> MQNLEAQVTGSLVAFPDVTQKALKEDEINLDSVLRGKFSTGRTSLAWLACGPQLEITNSVTGERISAYHFSGLTERPPVVVAVKEFTWQKKTGLLVGLVEAEGSVLCLYDIGISKVVKAVVLPGSVTAVEPIINHGGASASTQHLHQSLRWFFGVTAVVTDVGHVLLIDLCLDEVSSNQDELDASDLEVMSVIPTKIPKLREAATRERRHLCLQLAAPTGTTVSCLSYISRTNQLAVGYSDGYFSLWNMKTLRRDYHVQIEGGRVPVCAVAFQEPENDPRNCCYLWAVQSSESGGDVSLHLLQLAFSDRKCLASGQIMYELLEYCEERYSLDLSGSTLSLRGQSNNTKLLGCQTIEKFRVHGEREDGVHEVTSPDTSVSVFSWQVNTYGQGKPSVYLGVFDINRWYQAQMPDSLRSGQFLRNCSYFAFWSLEAVVNITTQDIIFDILVHERSLSRGIPPSYPPPEQFYYPSTYNFDATCLLNSGLIHFACTGFQKETLHFLKKSGSSLNEAIPDGYNRCLAAGLLAPKFTDVQASSLSQEEQLQAILAAAVETSSLGLLTSCIKRWTAEEQPRSAANLRFVLEWTWKKVTLTKQEFDRLCFRLFDGSCNFIDPHTLQSLQQCHLYFSNLTAVLNCFIAQAKEVTQQGAVDLTNKQSVTRLLTLYASVVLWFCRSGMLPDSSDETVQLTRPFYNYQVIQQYYSDQRKKLERLARGKWDTSSLMIDGLINQFGDRIQQLWSRDDNGTGKYPPANLHALLDVYLLENADEMSKHAITIYFLLDIMYSFPDKPDSSIESFPTAFFVPGSLIKLIQGFWLLDHNDYQNSVDCILNPASSRVMSWQHSQIIENLLCHGDSRQALRYLQVMKPVATTSKEVKLHMTVLLANRSILEAWNLQRLHSSRLNVEELLKHMYEMCQEMGLIEELLKLTFTDFEQGYLHKFLQTTGVQNQELLLVHHLQRANYISALQLNQSLKTNHLNDCDRRLRERSGARNAILDQYGKILPRVQRTLASERAKPYSLPSLVWREVARPKPLSTTAKQAAPGSIITKANFICNVLSKIKEVSTANEKREEYSPYQSMVSEEPTAPPLQDIDVPDAFFGTPINKSRRVSRLLDSVVHPVLMEPTPLTSSDTDNNQTPHKSPLLKTSSPLHSSLRRIAHMRSFAKASEFSLLETPLVVRKAKALAANTASSGYTSITPQSILRSSVRTTPLVSPSVSPGRSLTPPLRPKETKISFMELSFTRHAKAAHSSEGNLLAISPVLRSSPDAVWSVKGKVASFTQNTPVKKLDEIDASSSGIQEESQDEMEVSKEISNISVRSEQASLEYHDAPTPEDLENDEISGTTNSQPQVNEVHHQMEDGQLTEKPAELALTEMQEEFIDSEEREIEYISAPLNGPNALECMTAVPDIYLEDASQCILETPEGSSVSVTGEQECVSSAKDSESVISIHDSDDAHSNLSENDQDSEEIEENNLRVPTTVTRCEEFDLIETKDLEVELEEADSEKTNYKDIYPDATVQLGFTVESIEQRYTCELADRRETPSETDEIEGEHFETENNFSLVLEGDVTEEEILEPSSSKTDLELTRPPIAHQKLISENRENIENCETTEKIPANMSPLVDSDHESKTLETLPSEADLSVAEKVLKGTEEKDVPPEVHSEVVLESKLVGNAMMSLDSSESQEVIISQYDNVISIEKLEMTQEKMYGEKTEQINEGQVSPNRDQSTLVKPLTPRRSIRKSSKPADSSTDIIGNITLPTTPKRGLKKAKENVDTLKNSISVVPEEELTLGTRRITRKATLTALDNPEPLQIKEPPSGEDLQVQPSTPTRGRRGKVITSDDLKEPPSGEDLQVQPSTPTRGRRGRVITSDDLREPPPGEDLQVQPSTPTRGRRGRVITSDDIKESPSVEDLQVQPSTPTRGRRGKVITSDDIKEPPSVEDLQVQPSTPTRGRKGKVITSDDIKEPLSGEDLQVQPSTPTRGRKGKVITSDDIKEPLSEEVLQEQPSTPTRGRRGRVITSDGKGYECVEEKNALPLTPTRITRSKNILEPEKGISQIEPEKGISQIEPDKGLSQIEDTGETEHEVVTPRRGRRGKRVVNELVKHFERNSSQPNIKADTSPPVSPKKVSLRWTRTRSENQRINATEEQASKIQEDLSDTPRKRYKKSSNKMGFEETTDTVTEGAIVEDVQESLIISHLGKNPNTSIVRSARKTALPPVTEDHSEQPLLPPESHSKVHSSLAIADEENKTNTRTRSGNKSSVDVSAITFEFSTPKARTKKTAKGSAVPTELIPSTQYVFSPPSTRTRRATRANVSEAVI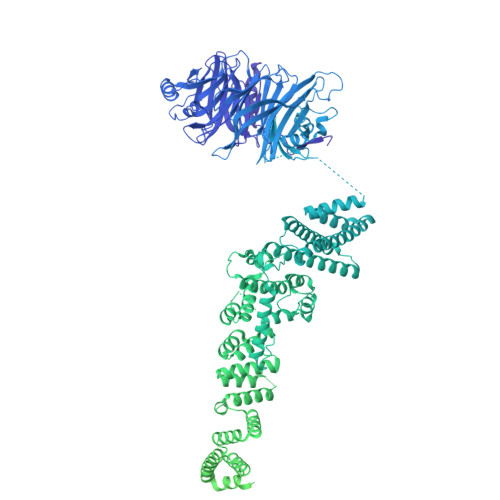EPQLQFQESCEIAETEVPEVPASKPRGRPPKHKAKAVTRVLKKPSWSTPPVEIKLISPPESPAVSETNTKTDSTEAKGAEKISVRRTRRRIIAKPVTRRKMR>MSLMKNILAIQSHVVYGHAGNSAAEFPMRRLGANVWPLNTVQFSNHTQYGKWTGCVMPPSHLTEIVQGIAAIDKLHTCDAVLSGYLGSAEQGEHILGIVRQVKAANPQAKYFCDPVMGHPEKGCIVAPGVAEFHVRHGLPASDIIAPNLVELEILCEHAVNNVEEAVLAARELIAQGPQIVLVKHLARAGYSRDRFEMLLVTADEAWHISRPLVDFGMRQPVGVGDVTSGLLLVKLLQGATLQEALEHVTAAVYEIMVTTKAMQEYELQ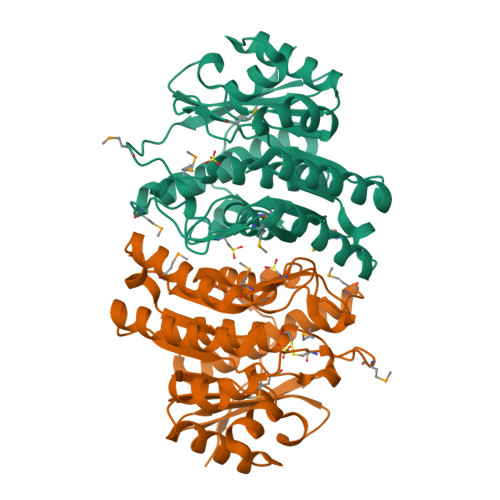VVAAQDRIAKPEHYFSATKLEGGSHHHHHH[4x]>WVQPITAQKPSLTLWLDDKMFTGLINTGADVTIIKLEDWPPNWPITDTLTNLRGIGQSNNPKQSSKYLTWRDKENNSGLIKPFVIPNLPVNLWGRDLLSQMKIMMAS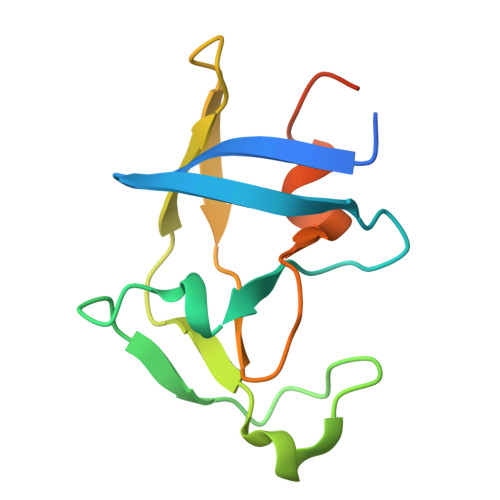PNDIVTA[2x]>[10x]EAEAADRADILYNIRQTSRPDVIPTQRDRPVAVSVSLKFINILEVNEITNEVDVVFWQQTTWSDRTLAWDSSHSPDQVSVPISSLWVPDLAAYNAI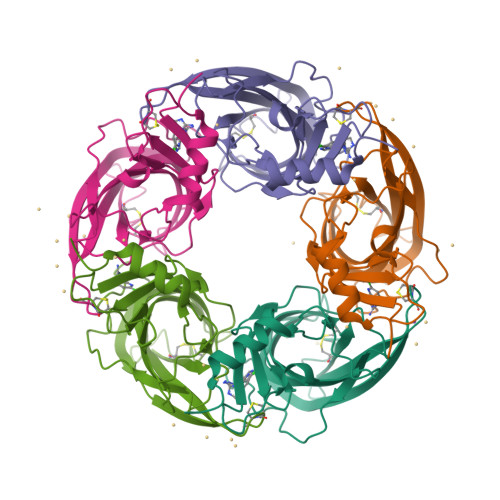SKPEVLTPQLARVVSDGEVLYMPSIRQRFSCDVSGVDTESGATCRIKIGSWTHHSREISVDPTTENSDDSEYFSQYSRFEILDVTQKKNSVTYSCCPEAYEDVEVSLNFRKKGRSEIL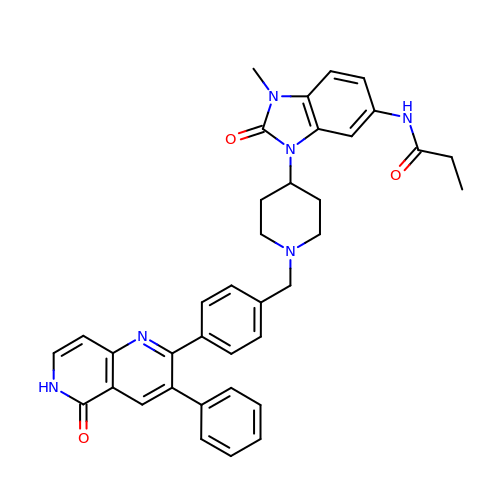~{N}-[1-methyl-2-oxidanylidene-3-[1-[[4-(5-oxidanylidene-3-phenyl-6~{H}-1,6-naphthyridin-2-yl)phenyl]methyl]piperidin-4-yl]benzimidazol-5-yl]propanamide | C37 H36 N6 O3 | NOAOWOIAXARUHL-UHFFFAOYSA-N> GPPVVEEDDVVGFDDEAQTVIDRLL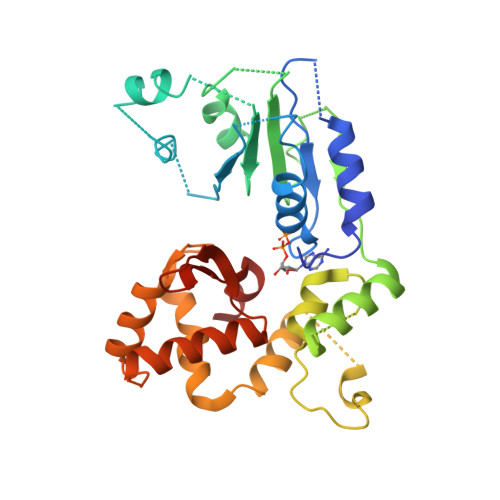EGSGDLEVIPVVGMPGLGKTTLATKIFKHPKIEYEFFTRLWLYVSQSYKTRELYLNIISKFTGNTKHCRDMSEKDLALKVQEILEEGGKYLIVLDDVWSTDAWDRIKIAFPKNDKGNRVLLTTRDHRVARYCNRSPHDLKFLTDEESWILLEKRAFHKAKCLPELETNGKSIARKCKGLPLAIVVIAGALIGKSKTIKEWEQVDQSVGEHFINRDQPNSCDKLVRMSYDVLPYDWKACFLYFGTFPRGYLIPARKLIRLWIAEGFIQYRGDLSPECKAEEYLNELVNRNLVMVMQRTVDGQIKTCRVHDMLYEFCWQEATTE>[3x]MQSDTQEANDIVTLANLQYNGSTPADAFETKVTNIIDRLNNNGIHINNKVACQLIMRG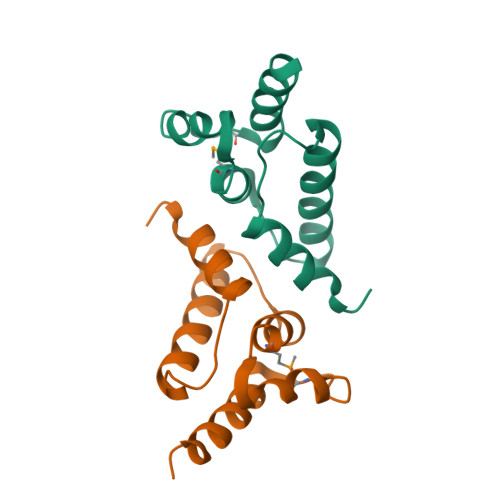LSGEYKFLRYTRHRHLNMTVAELFLDIHAIYEEQQGSRNPLEHHHHHH> 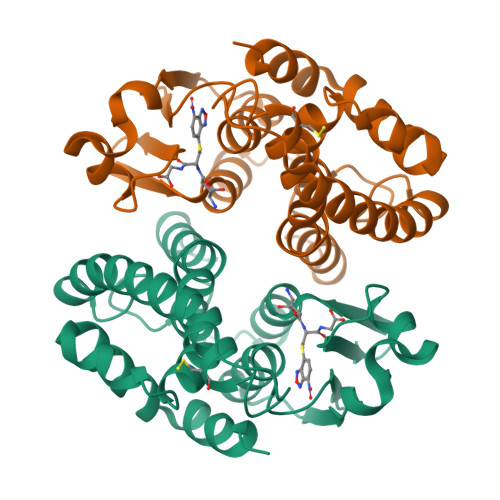MAPVKVFGPAMSTNVARVTLCLEEVGAEYEVVNIDFNTMEHKSPEHLARNPFGQIPAFQDGDLLLWESRAISKYVLRKYKTDEVDLLRESNLEEAAMVDVWTEVDAHTYNPALSPIVYQCLFNPMMRGLPTDEKVVAESLEKLKKVLEVYEARLSKHSYLAGDFVSFADLNHFPYTFYFMATPHAALFDSYPHVKAWWDRLMARPAVKKIAATMVPPKA>SNAQENQVHIWAV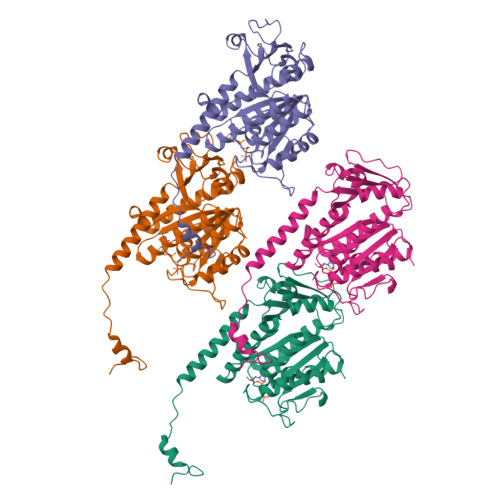GGCGGEIGSAFEGEVAKGLHSMTYVDTSRANLRDSTLGDDHIYIFKDAAGRELDGSGKKRDENAELICSQIPGILNKHTPGKFNIVVFSLSGGSGSVAGPALVANLLERGERVVCCIVASFDDERQTINADRTFKGLMAAAEGLKRPVIVSYHMNGENGKSEQDVNLDVQVVISQLCVLFSGENRRLDSADLENFLNHPRVTGLEPTITELNTFMGYEWTKENDSPIAFCTLYPKDATKVMGVSAIYSCDGFVPESSPIREATSFVLSTDRLGGIIKQIADEAKRYIEHRNARQQAPKVGDETVAEAKNSGFLLF[4x]> NVQHQLAQFQQLQQQAQAISVQKQTVEMQINETQKALEELSRAADDAEVYKS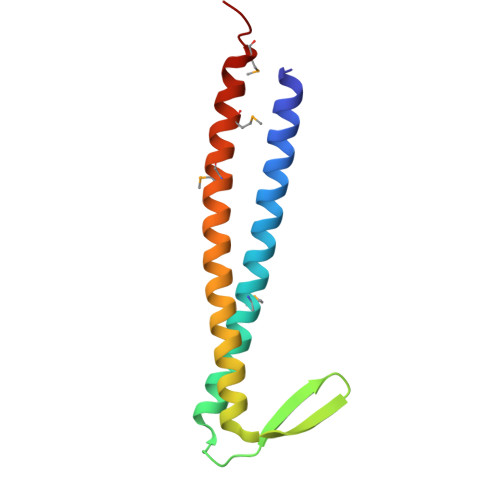SGNILIRVAKDELTEELQEKLETLQLREKTIERQEERVMKKLQEMQVNIQEAMKGAG> GREEAPNAEADILSCRLPGVVMTTSPIITNNSINIFVGPGTDISSLAPEFTLTPGATIDPPSGTARDFHSPQQYTVTAADGFWKKKYTVSVIDTELATIYNF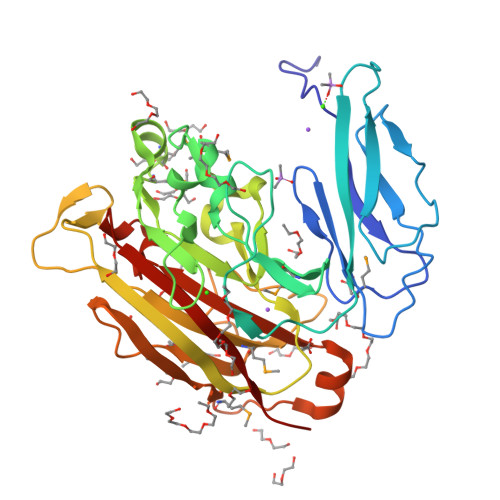EDTLGGQKYYIFVEREGEKVVMEWASGNAGYAMTGVPKTADDYPTFQFANGKTGKCLSLVTRSTGFFGSIMGMPIAAGNLFIGSFDVGNAMSNPLKATKFGLPFRHIPTYLAGYYKYKAGDQFTEGGKPVSGKRDICDIYAIMYETSESVPTLDGTNAFTSPNLVSIARIDDAKETDEWTYFKLPFHMLSGKYIDKEKLTAGKYNVAIVFTSSLEGDHFNGAIGSTLLIDEVELIYRSED2-[[(2~{R},3~{R},4~{R})-2-(hydroxymethyl)-3-oxidanyl-3,4-dihydro-2~{H}-pyran-4-yl]oxymethyl]quinoline-7-carboxylic 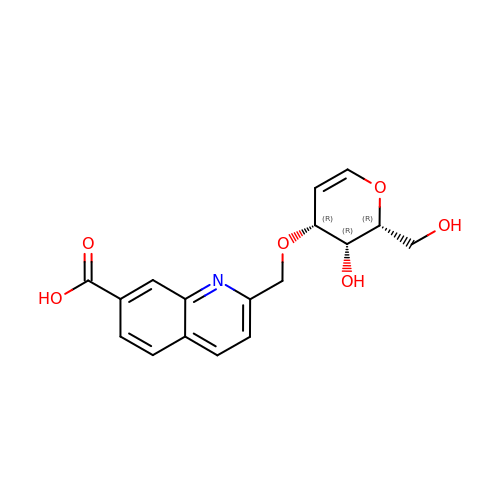acid | C17 H17 N O6 | ZGVBVJVFIXTFPT-BZUAXINKSA-N(3~{S})-2,2-bis(oxidanyl)-3-(phenylmethylsulfanyl)-3,4-dihydro-1,2-benzoxaborinin-2-ium-8-carboxylic acid | C16 H16 B O5 S | 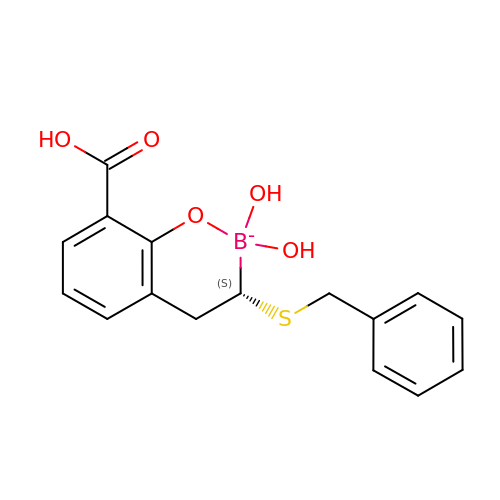NCOFNSDHLWCKKT-CQSZACIVSA-N>[5x]MSVTVKRIIDNTVIVPKLPANEDPVEYPADYFRKSKEIPLYINTTKSLSDLRGYVYQGLKSGNVSIIHVNSYLYGALKDIRGKLDKDWSSFGINIGKAGDTIGIFDLVSLKALDGVLPDGVSDASRTSADDKWLPL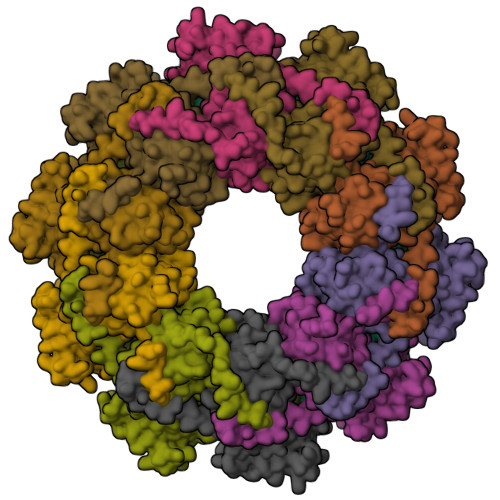YLLGLYRVGRTQMPEYRKKLMDGLTNQCKMINEQFEPLVPEGRDIFDVWGNDSNYTKIVAAVDMFFHMFKKHECASFRYGTIVSRFKDCAALATFGHLCKITGMSTEDVTTWILNREVADEMVQMMLPGQEIDKADSYMPYLIDFGLSSKSPYSSVKNPAFHFWGQLTALLLRSTRARNARQPDDIEYTSLTTAGLLYAYAVGSSADLAQQFCVGDNKYTPDDSTGGLTTNAPPQGRDVVEWLGWFEDQNRKPTPDMMQYAKRAVMSLQGLREKTIGKYAKSEFDK>MASHHHHHHMASNTVKITISFDNYAYLEGFQTLWGFSCFVETDETTFLFDTGSNGRVLLQNMQQLDIDLKKAEALILSHPHWDHIGGVDSVLEVHPQMHLFVPNSLSKHLIRDLNAQTLGVTVINESPQQLLPSVYSTGVMGDIGEQSIVIDTEKGLVVITGCAHPGIEHIAARSIEMLQKPIYLLMGGFHLMYENTA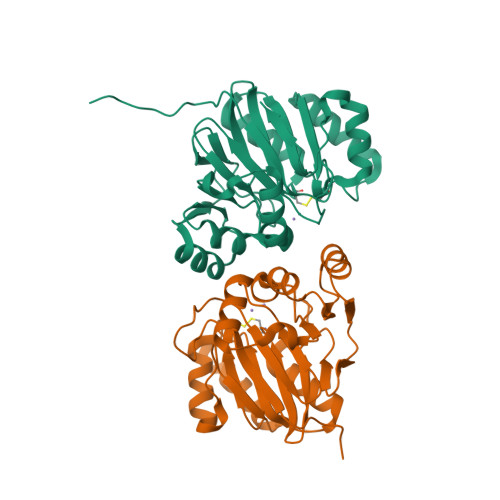RISEVIETLDELGIQNVCPTHCSGDLAISMFKSHFGDRCLQGGIGRVITI[2x]> KDDILCMASHDKGETWGTKIVIKYDNYKLGVQYFFLRPYISKNDLSFHFYVGDNINNVKNVNFIECTHEKDLEFVCSNRDFLKDNKVLQDVSTLNDEYIVSYGNDNNFAECYIFFNNEN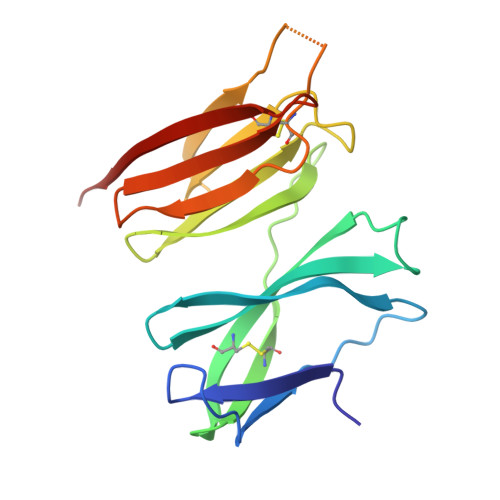SILIKPEKYGNTTAGCYGGTFVKIDEQRTLFIYSSSQGIYNIHTIYYANYE>[4x]MRGSHHHHHHGSSEPLILDAPNADACIIWLHGLGADRTDFKPVAEALQMVLPS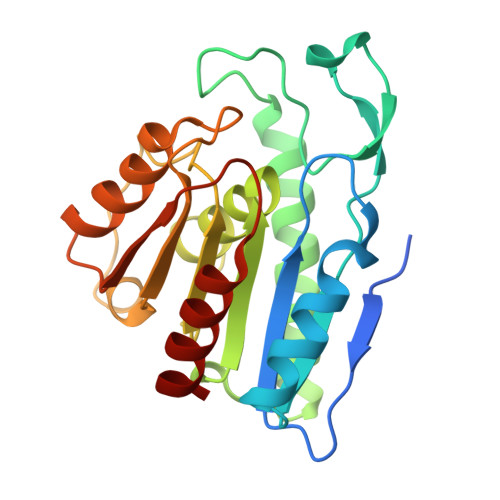TRFILPQAPSQAVTVNGGWVMPSWYDILAFSPARAIDEDQLNASADQVIALIDEQRAKGIAAERIILAGFSQGGAVVLHTAFRRYAQPLGGVLALSTYAPTFDDLALDERHKRIPVLHLHGSQDDVVDPALGRAAHDALQAQGVEVGWHDYPMGHEVSLEEIHDIGAWLRKRL>MVKLENSRKPEKISNKNIPMSDFVVNLDHGDPTAYEEYWRKMG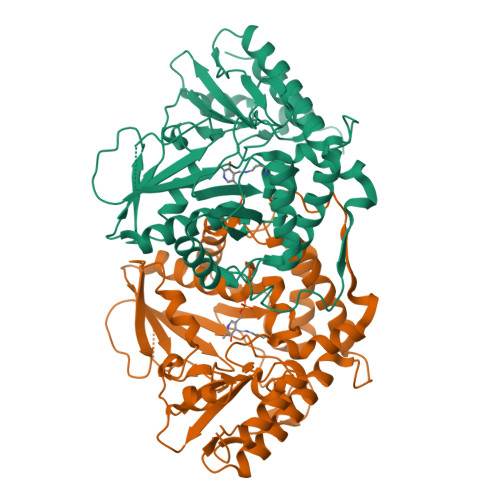DRCTVTIRGCDLMSYFSDMTNLCWFLEPELEDAIKDLHGVVGNAATEDRYIVVGTGSTQLCQAAVHALSSLARSQPVSVVAAAPFYSTYVEETTYVRSGMYKWEGDAWGFDKKGPYIELVTSPNNPDGTIRETVVNRPDDDEAKVIHDFAYYWPHYTPITRRQDHDIMLFTFSKITGHAGSRIGWALVKDKEVAKKMVEYIIVNSIGVSKESQVRTAKILNVLKETCKSESESENFFKYGREMMKNRWEKLREVVKESDAFTLPKYPEAFCNYFGKSLESYPAFAWLGTKEETDLVSELRRHKVMSRAGERCGSDKKHVRVSMLSREDVFNVFLERLANMKLIKSIDL[6x]> MGSAWSHPQFEKSSGLEVLFQGPHMSRNLKHERFQSLSFPHTKEMMKIFHKKFGLHNFRTNQLEAINAALLGEDCFILMPTGGGKSLCYQLPACVSPGVTVVISPLRSLIVDQVQKLTSLDIPATYLTGDKTDSEATNIYLQLSK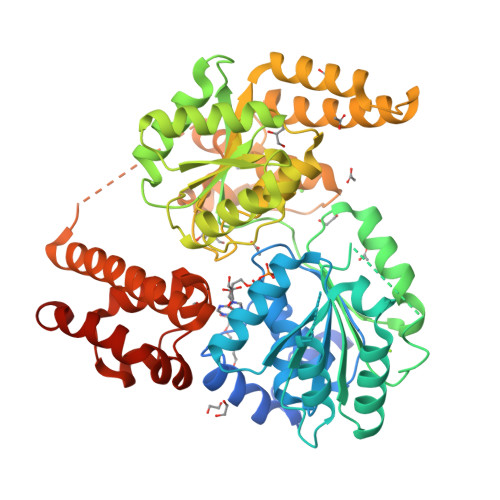KDPIIKLLYVTPEKICASNRLISTLENLYERKLLARFVIDEAHCVSQWGHDFRQDYKRMNMLRQKFPSVPVMALTATANPRVQKDILTQLKILRPQVFSMSFNRHNLKYYVLPKKPKKVAFDCLEWIRKHHPYDSGIIYCLSRRECDTMADTLQRDGLAALAYHAGLSDSARDEVQQKWINQDGCQVICATIAFGMGIDKPDVRFVIHASLPKSVEGYYQESGRAGRDGEISHCLLFYTYHDVTRLKRLIMMEKDGNHHTRETHFNNLYSMVHYCENITECRRIQLLAYFGENGFNPDFCKKHPDVSCDNCCKTKGSGGSKALVAKVSQREEMVKKCLGELTEVCKSLGKVFGVHYFNIFNTVTLKKLAESLSSDPEVLLQIDGVTEDKLEKYGAEVISVLQKYSEWTSPAEDSSPG> MFLKVRAEK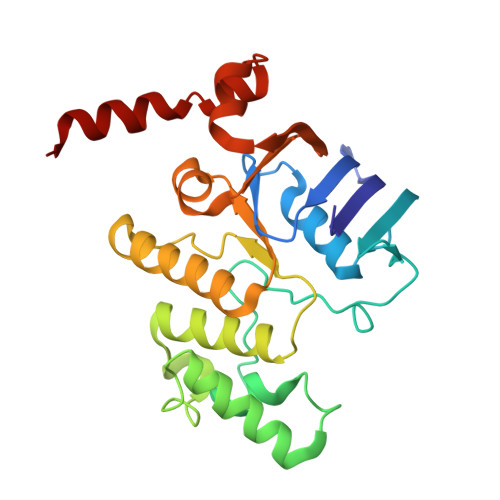RLGNFRLNVDFEMGRDYCVLLGPTGAGKSVFLELIAGIVKPDRGEVRLNGADITPLPPERRGIGFVPQDYALFPHLSVYRNIAYGLRNVERVERDRRVREMAEKLGIAHLLDRKPARLSGGERQRVALARALVIQPRLLLLDEPLSAVDLKTKGVLMEELRFVQREFDVPILHVTHDLIEAAMLADEVAVMLNGRIVEKGKLKELFSAKNGEVAEFLSARNLLLKVSKILD> GPLGSLFRSLVGTSRAIQQVRQMMQQVADTDASVLILGESGTGKEVVARNLHYHSKRREGPFVPVNCGAIPAELLESELFGHEKGAFTGAITSRAGRFELANGGTLFLDEIGDMPLPMQVKLLRVLQERTFERVG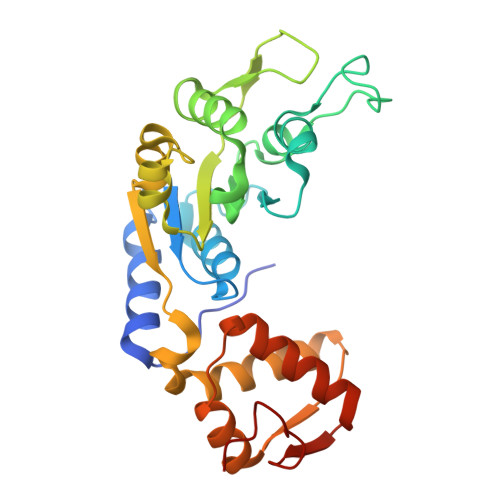SNKTQNVDVRIIAATHKNLEKMIEDGTFREDLYYRLNVFPIEMAPLRERVEDIALLLNELISRMEHEKRGSIRFNSAAIMSLCRHDWPGNVRELANLVERLAIMHPYGVIGVGELPKKFRHVDD> MNIDVEFH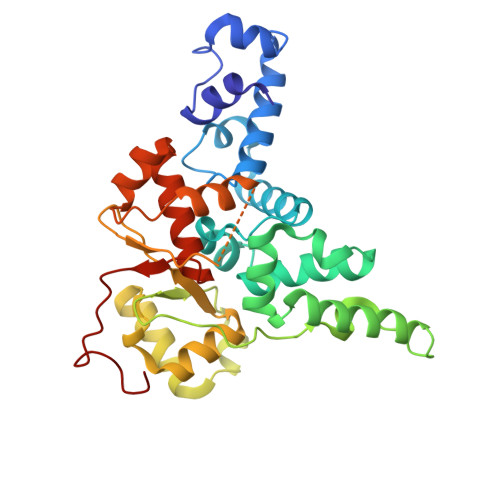IRHNYPWNKLPANVRQSLGNSQREYEKQVVLYSIRNQLRYRNNLVKHVKKDERRYYEELLKYSRDHLMLYPYHLSDIMVKGLRITPFSYYTGIMEDIMNSEKSYDSLPNFTAADCLRLLGIGRNQYIDLMNQCRSSKKFFRRKTARDLLPIKPVEIAIEAWWVVQAGYITEDDIKICTLPEKCAVDKIIDSGPQLSGSLDYNVVHSLYNKGFIYLDVPISDDSCIAVPPLEGFVMNRVQGDYFETLLYKIFVSIDEHTNVAELANVLEIDLSLVKNAVSMYCRLGFAHKKGQVINLDQLHSSWK> MQKIALCITGASGVIYGIKLLQVLEELDFSVDLVISRNAKVVLKE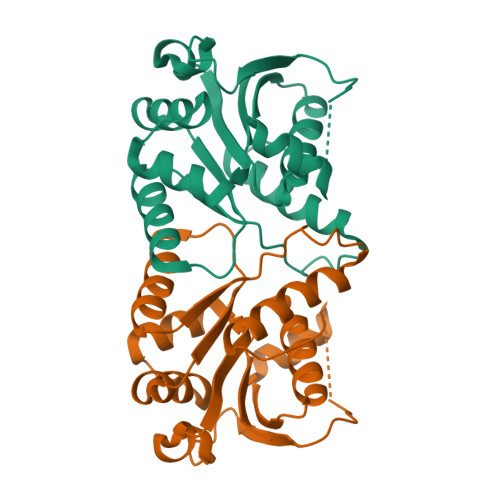EHSLTFEEVLKGLKNVRIHEENDFTSPLASGSRLVHYRGVYVVPCSTNTLSCIANGINKNLIHRVGEVALKERVPLVLLVREAPYNEIHLENMLKITRMGGVVVPASPAFYHKPQSIDDMINFVVGKLLDVLRIEHNLYKRWRG>MKVISFLNPKGGSGKTTAVINIATALSRSGYNIAVVDTDPQMSLTNWSKAGKAAFDVFTAASEKDVYGIRKDLADYDFAIVDGAGSLSVITSAAVMVSDLVIIPVTPSPLDFSAAGSVVTVLEAQAYSRKVEARFLITRKIEMATMLNVLKESIKDTGVKAFRTAITQRQVYVKSILDGDSVFESSDGAAKGEIEILTKEIVRIFEATHHHHHH[4x];>[4x]KAHTSVKKMTFGENRDLER

Walker-box partition systems are ubiquitous in nature and mediate the segregation of bacterial and archaeal DNA. DNA segregation by these systems requires, minimally, a centromere site located on the DNA to be segregated; a nucleotide triphosphatase (NTPase), typically called ParA; and a centromere-binding protein (CBP), termed ParB. A distinguishing feature of the Walker-box systems is that their ParA NTPases bind and use nonspecific nucleoid DNA (nsDNA) as a substratum to equipartition replicated DNA. In these systems, ParA–ATP binds nucleoid DNA and uses it as a substratum to deliver ParB-attached cargo DNA, and ParB drives ParA dynamics, allowing ParA progression along the nucleoid.

Crystals were obtained of the complex formed between the TP228 plasmid ParA and ParB proteins (also called ParF and ParG) in the presence of AMPPNP. TP228 can replicate in low copy number in E. coli, and its retention depends on the type I Walker-box cassette that includes the small 206-residue Walker-box ParA protein and the 76-residue ParB protein, which is composed of an N-terminal disordered region that binds ParA followed by a ribbon–helix–helix DNA-binding motif. Crystals of the TP228 ParA–AMPPNP–ParB complex took 6 mo to grow, and the structure was solved to 3.65 Å. The structure revealed density for only ∼15 N-terminal ParB residues, consistent with the subsequent finding that it had degraded during the extended crystallization process. In the structure, the ParB fragments dock as helices within the crevice at the ParA dimer interface. The formation of the ParB–ParA complex buries ∼450 Å2 of protein surface from solvent, consistent with data indicating that the ParA–ParB interaction is weak. Strikingly, the ParB helices interact specifically with the ParA subunit arrangement found in the nucleotide sandwich dimer state; comparison of the ParA–ParB and ParA–DNA structures shows that ParB cannot dock in the dimer interface of the conformation that ParA adopts when bound to DNA without clash. Thus, the structure indicates that ParB binding stabilizes the ParA nucleotide sandwich dimer conformation and not the DNA-binding state. Although the ParA–AMPPNP–ParB structure is low resolution, the best fit to the ParB helical density places ParB hydrophobic residues pointing into the ParA dimer interface with Gly16 juxtaposed next to ParA residues Val1149 and Pro109. While the Arg19 side chain position is equivocal due to the low resolution of the current structure, this fit positions ParB Arg19 proximal to the AMPPNP γ-phosphate in the ParA active site, suggesting that it could aid in the stabilization of the transition state in which the γ-phosphate becomes partially hydrolyzed.> MATLRRLREAPRHLLVCEKSNFGNHKSRHRHLVQTHYYNYRVSFLIPECGILSEELKNLVMNTGPYYFVKNLPLHELITPEFISTFIKKGSCYALTYNTHIDEDNTVALLPNGKLILSLDKDTYEETGLQGHPSQFSGRKIMKFIVSIDLMELSLNLDSKKYERISWSFKEKKPLKFDFLLAWHKTGSEESTMMSYFSKYQIQEHQPKVALSTLRDLQCPVLQSSELEGTPEVSCRALELFDWLGAVFSNVDLNNEPNNFISTYCCPEPSTVVAKAY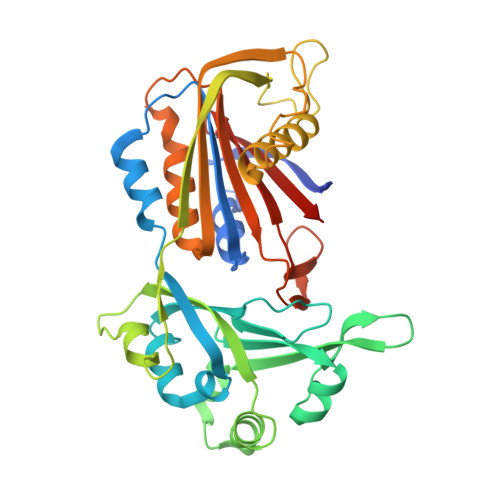LCTITGFILPEKICLLLEHLCHYFDEPKLAPWVTLSVQGFADSPVSWEKNEHGFRKGGEHLYNFVIFNNQDYWLQMAVGANDHCPP>[4x]MYRLLNKTAVITGGNSGIGLATAKRFVAEGAYVFIVGRRRKELEQAAAEIGRNVTAVKADVTKLEDLDRLYA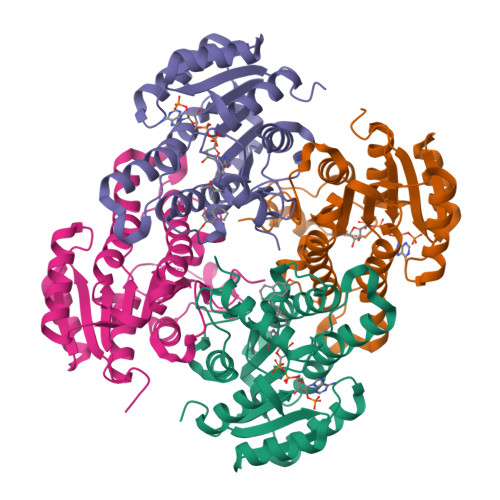IVREQRGSIDVLFANSGAVEQKTLEEITPEHYDRTFDVNVRGLIFTVQKALPLLRDGGSVILTSSVAGVLGLQAHDTYSAAKAAVRSLARTWTTELKGRSIRVNAVSPGAIDTPSLENQVSTQEEADELRAKAAAATPLGRVGRPEELAAAVLFLASDDSSYVAGIELFVDGGLTQV>AKVNIKPLEDKILVQANEAETTTASGLVIPDTAKEKPQEGTVVAVGPGRWDEDGEKRIPLDVAEGDTVIYSKYGGTEIKYNGEEYLILSARDVLA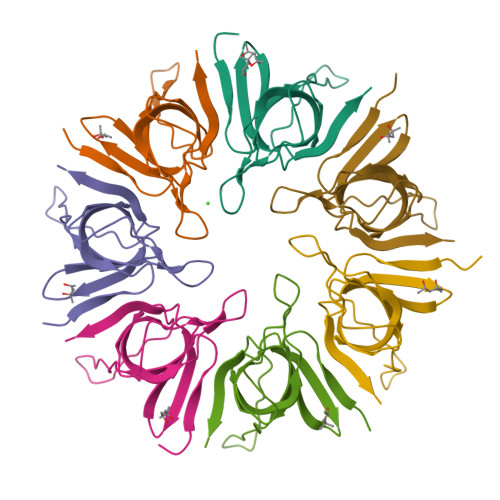VVSK[14x]2-azanyl-9-[(4-bromanyl-2-fluoranyl-phenyl)methyl]-6-chloranyl-purin-8-ol 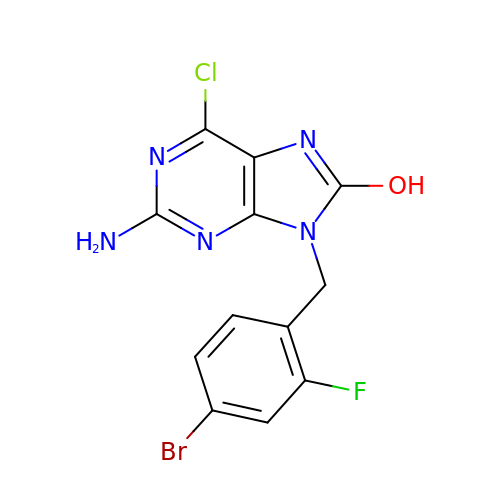| C12 H8 Br Cl F N5 O | CCUHAWKQXDIYIR-UHFFFAOYSA-N>QGSYDYDLIVIGGGSAGLACAKEAVLNGARVACLDFVKPTPTLGTKWGVGGTCVNVGCIPKKLMHQASLLGEAVHEAAAYGWNVDDKIKPDWHKLVQSVQNHIKSVNWVTRVDLRDKKVEYINGLGSFVDSHTLLAKLKSGERTITAQTFVIAVGGRPRYPDIPGAVEYGITSDDLFSLDREPGKTLVVGAGYIGLECAGFLKGLGYEPTVMVRSIVLRGFDQQMAELVAASMEERGIPFLRKTVPLSVEKQDDG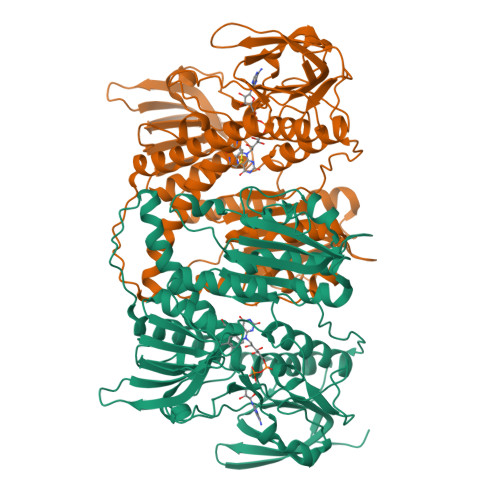KLLVKYKNVETGEESEDVYDTVLWAIGRKGLVDDLNLPNAGVTVQKDKIPVDSQEATNVANIYAVGDIIYGKPELTPVAVLAGRLLARRLYGGSTQRMDYKDVATTVFTPLEYACVGLSEEDAVKQFGADEIEVFHGYYKPTEFFIPQKSVRYCYLKAVAERHGDQRVYGLHYIGPVAGEVIQGFAAALKSGLTINTLINTVGIHPTTAEEFTRLAITKRSGLDPTP[2x]> STRDYEIQRERIELGRCIGEGQFGDVHQGIYMSPENPALAVAIKTCKNCTSDSVREKFLQEALTMRQFDHPHIVKLIGVITENPVWIIMELCTLGELRSFLQVRKYSLDLASLILYAYQLSTALAYLESKRFVHRDIAARNVLVSSNDCVKLGDFGLSRYMEDSTYYKASKGKLPIKWMAPESINFRRF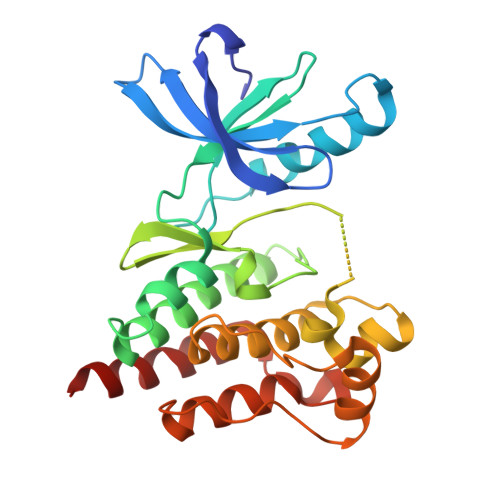TSASDVWMFGVCMWEILMHGVKPFQGVKNNDVIGRIENGERLPMPPNCPPTLYSLMTKCWAYDPSRRPRFTELKAQLSTILEEEKLQ>[4x]AHMEQEERKRFFNDDLDTSGGSSSSLVPRGSGGSGGSPKFQNLTRFKKICQLVKQWVAETLGDGGPHEKDVKLFVKYLI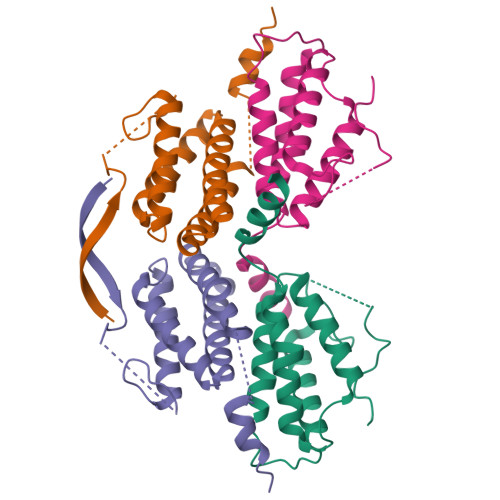KLCDSNRVHLVLHLSNLISRELNLCAFLNQDHSGFQTWERILLNDIIPLLNRNKHTYQTVRKLDMDFEV> MDQKASYFINEKLFTEVKPVLFTDLIHHLKIGPSMAKKLMFDYYKQTTNAKYNCVVICCYKD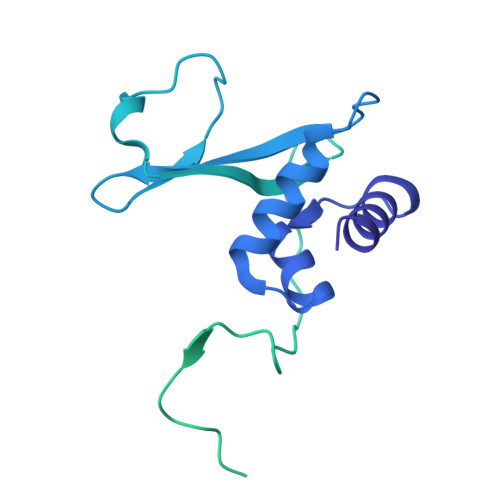QTIKIIHDLSNIPQQDSIIDCFIYAFNPMDSFIPYYDIIDQKDCLTIKNSYELKVSESSKIIERTKTLEEKSKPLVRPTARSKTTPEETTGRKSKSKDMGLRSTALLAKMKKDRDDKETSRQNELRKRKEENLQKINKQNPEREAQMKELNNLFVEDDLDTEEVNGGSKPNSPKETDSNDKDKNNDDLEDLLETTAEDSLMDVPKIQQTKPSETEHSKEPKSEEEPSSFIDEDGYIVTKRPATSTPPRKPSPVVKRALSSSKKQETPSSNKRLKKQGTLESFFKRKAK> QQCNGIYIWKIGNFGMHLKCQEEEKPVVIHSPGFYTGKPGYKLCMRLHLQLPTAQRCANYISLFVHTMQGEYDSHLPWPFQGTIRLTILDQSEAPVRQNHEEIMDAKPELLAFQRPTIPRNPKGFGYVTFMHLEALRQRTFIKDDTLLVRCEVSTR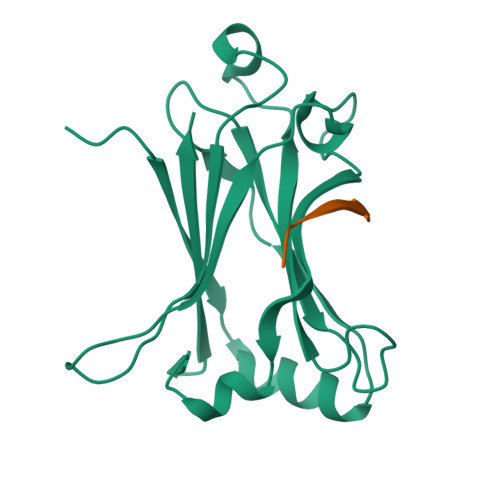FDLE;> QMPTEDEY>GAPSQGATANAETQTTIPLGDTSQNALDWPGVYEGVLPCASCEGIQTTLTLQADNSFELKSIYLGKDESIFKVAGKFDWDSNGSKITLSDGSKYLVGENQLLMLDTEGNRITGGLAE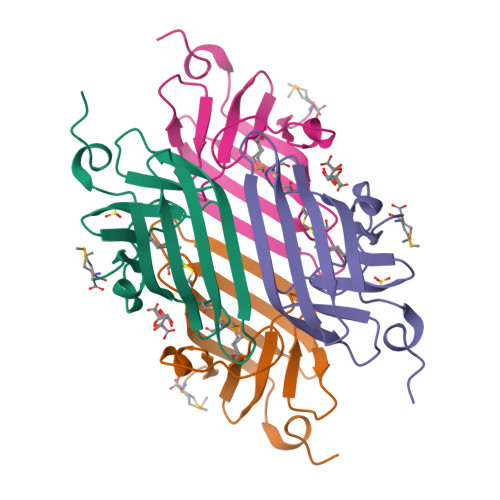HYILKKKGM[2x]> ACDY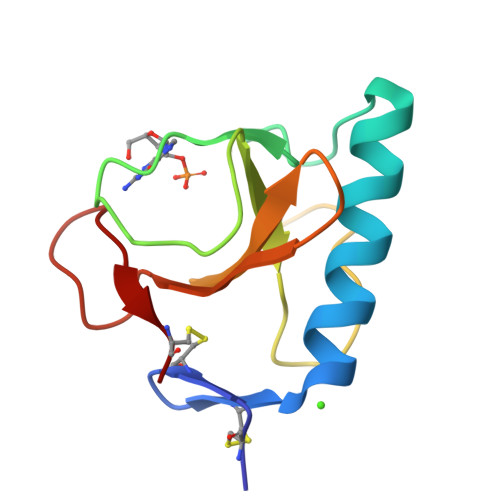TCGSNCYSSSDSSTAQAAGYKLHEDGETVGSNSYPHKYNNYEGFDFSVSSPYYEWPILSSGDVYSGGSPGADRVVFNENNQLAGVITHTGASGNNFVECT{4-[(N-{3-[5-chloro-2-(1H-tetrazol-1-yl)phenyl]propanoyl}-L-phenylalanyl)amino]phenyl}acetic acid | C27 H25 Cl N6 O4 | 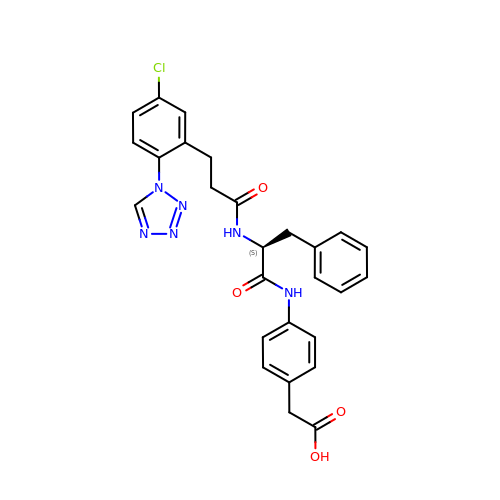WNOHYEPACJOGFG-QHCPKHFHSA-N>[26x]AVTGQVDVKLNISTGCTVGGSQT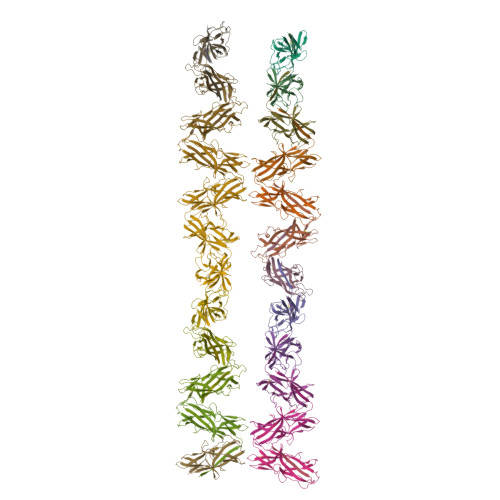EGNMNKFGTLNFGKTSGTWNNVLTAEVASAATGGNISVTCDGTDPVDFTVAIDGGERTDRTLKNTASADVVAYNVYRDAARTNLYVVNQPQQFTTVSGQATAVPIFGAIAPNTGTPKAQGDYKDTLLVTVNF>[2x]SLFELGKMILQETGKNPAKSYGAYGCNCGVLGRGKPKDATDRCCYVHKCCYKKLTGCNPKKDRYSYSWKDKTIVCGENNPCLKELCECDKAVAICLRENLGTYNKLYRYHLKPFCKKADDC

A subgroup of PLA2s, known as PLA2-like proteins,is catalytically inactive due to lack of Ca2+ coordination related to natural mutationsof its primary structure; however, it is still able to induce a drastic local myonecrosis[8–10]. The most studied PLA2-like proteins are the Lys49-PLA2s, in which the mutations Asp49→Lys and Tyr28→Asn impair the Ca2+ coordination. In this work, we report functional (neuromuscular-blocking and muscle-damage activities) and crystallographicexperiments aimingto studythe possible inhibitory effects of AA and CA onPrTX-I, a Lys49-PLA2 isolated from Bothropspirajai snake venom. The final models are of a stereochemical quality expected for structures with the same resolution, as indicated by r.m.s.d bonds, r.m.s.d. angles and Ramachandran plot analyses. Both structures have seven disulfide bridges in each monomer with the following structural features: (i) an N-terminal α-helix; (ii) a “short” helix; (iii) a Ca2+ binding loop; (iv) two anti-parallel α-helices (2 and 3); (v) two short strands of an anti-parallel β-sheet (β-wing); and (vi) a C-terminal loop, similar to all other class II PLA2s.

The inspection of the 2ǀFobsǀ-ǀFcalcǀ electronic density mapof the PrTX-I/CA structure revealed the presence of four CA molecules establishing hydrogen bonds in monomer A with Lys15 and Arg118 and by water molecules with Ile82 and Lys100. In monomer B, CA molecules establish hydrogen bonds with Lys20 and Arg118 by water molecules with Gly15, Asn17 and Ser21. Moreover, CA molecules establish hydrophobic contacts with Lys20, Lys115, Ile104, Arg107, Glu108 and Leu121 in monomer A and with Lys15, Lys20 and Lys115 in monomer B. In addition,three PEG 4000 moleculeswere noted in the PrTX-I/CA structure,with two PEGs inside the hydrophobic channels from both monomersand the third PEG moleculeinteracting with Lys7 on monomer B. The PEG molecules found in these sites are found in other Lys49-PLA2s structures. Finally, in the PrTX-I/CA structure, a sulfate molecule establishedhydrogen bonds with Arg33 in monomer A, similarly to sulfate ions found in other Lys49-PLA2s structures. In the PrTX-I/CA crystal structure, four CA molecules interact with the protein. Two of them interact with Lys20, Lys115 and Arg118 residues for both monomers by hydrogen bonds and hydrophobic interactions. Regarding the other CA molecules, an interaction with Gly15, Asn17, Ser21 and Leu121 residues close to the MDiS region was observed, suggesting that this CA molecule may also bind to the membrane disruption site of PrTX-I. The fourth CA molecule interacts with Lys100 and Glu108 residues butno function has beenassignedto these residues; thus,the binding of this molecule can be attributed to a non-specific interaction. On the other hand, light microscopy analysis of muscle preparations submitted to myographic experiments showed that CA protected against the myotoxic effect induced by PrTX-I by 40% and 65% (PrTX-I/CA at ratios of 1:1 and 1:5, respectively).>[2x]MRKIVVAAIAVSLTTVSITASASADPSKDSKAQVSAAEAGITGTWYNQLGSTFIVTAGADGALTGT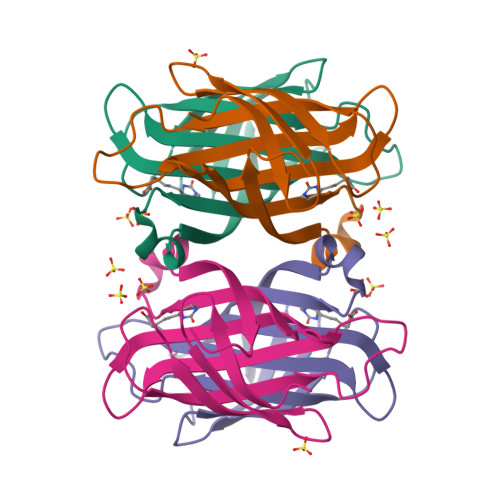YVTARGNAESRYVLTGRYDSAPATDGSGTALGWTVAWKNNYRNAHSATTWSGQYVGGAEARINTQWLLTSGTTEANAWKSTLVGHDTFTKVKPSAASIDAAKKAGVNNGNPLDAVQQ>MKSKFKLTTAAAMLGLMVLAGGAQAQDKPREVLTGGHSVSAPQENRIYVMDSVFMHLTESRVHVYDYTNGKFLGMVPTAFNGHVQVSNDGKKIYTMTTYHERITRGKRSDVVEVWDADKLTFEKEISLPPKRVQGLNYDGLFRQTTDGKFIVLQNASPATSIGIVDVAKGDYVEDVTAAAGCWSVIPQPNRPRSFMTICGDGGLLTINLGEDGKVASQSRSKQMFSVKDDPIFIAPALDKDKAHFVSYYGNVYSADFSGDEVKVDGPWSLLNDEDKAKNWVPGGYNLVGLHRASGRMYVFMHPDGKEGTHKFPAAEIWVMDTKTKQRVARIPGRDALSMTIDQQRNLMLTLDGGNVNVYDISQPEPKLLRTIEGAAEASLQVQFHPVGGV[2x];>[2x]AGGGGSSSGADHISLNPDLANEDEVNSCDYWRHCAVDGFLCSCCGGTTTTCPPGSTPSPISWIGTCHNPHDGKDYLISYHDCCGKTACGRCQCNTQTRERPGYEFFLHNDVNWCMANENSTFHCTTSVLVGLAKN;>[2x]ACDVSIEGNDSMQFNTKSIVVDKTCKEF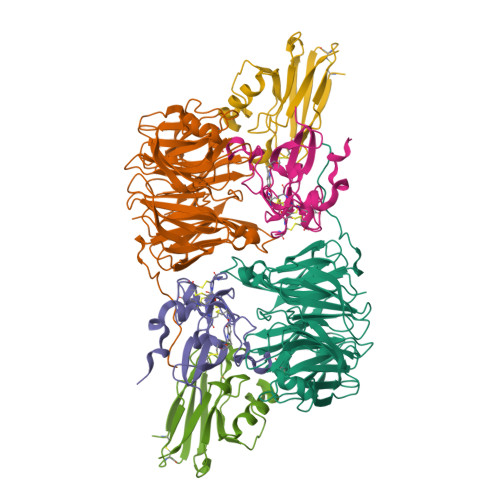TINLKHTGKLPKAAMGHNVVVSKKSDESAVATDGMKAGLNNDYVKAGDERVIAHTSVIGGGETDSVTFDVSKLKEGEDYAFFCSFPGHWSIMKGTIELGS>[2x]AAESGVSRPVPQLKRTTMRILIGLLVQNPELATLVPPLENLDENKLPGLGLFRELVNTCLSQPGL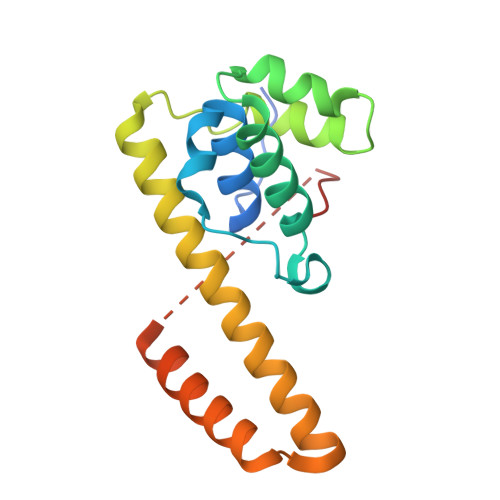TTGQLLEHYRGTNNAATLEKLSMWDDIADKNIAEQTFTDSLNHMFDSLLELRQEELIARERTHGLSNEERLELWTLNQELAKKTRESGSIGSMDFDDDIPF>VDQADDAAIQQTLAKMGIKSSDIQPAPVAGMKTVLTNSGVLYITDDG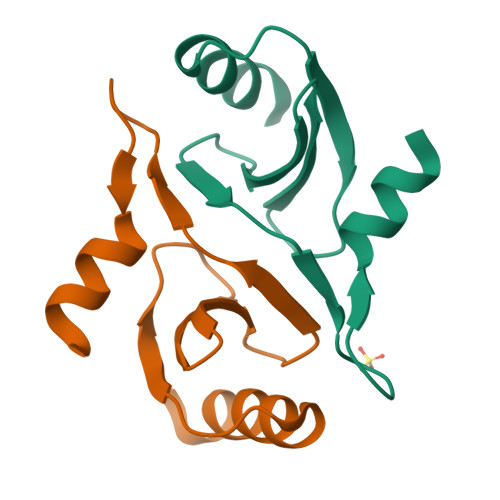KHIIQGPMYDVSGTAPVNVTNKMLLKQL[2x]> MDPSVTLWQFLLQLLREQGNGHIISWTSRDGGEFKLVDAEEVARLWGLRKNKTNMNYDKLSRALRYYYDKNIIRKV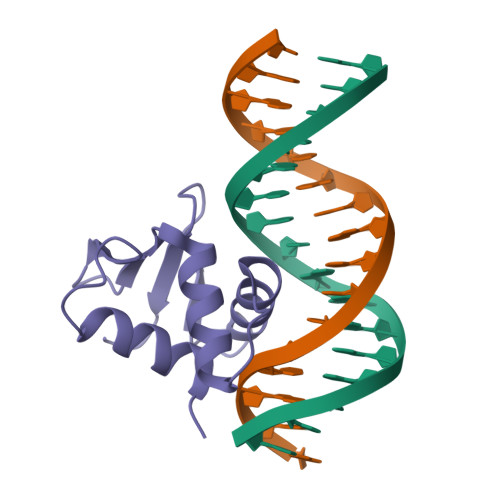SGQKFVYKFVSYPEVAGC>[4x]UGGAAGAAAUCGAAGAAGAUGAAGAACGCG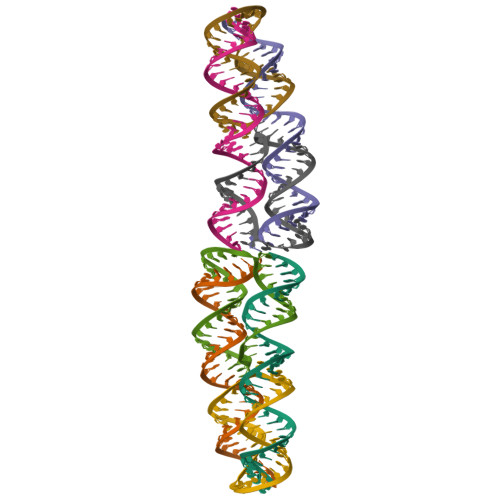AAGAAC;>[4x]AUCUUCUUCGAUUUCUUCCAGUUCUUCGCGUUCUUC> MSQIMYNYPAMLAHAAEMNTYSGALHAVGADIAAEQHALASAWQGDTGMTYQA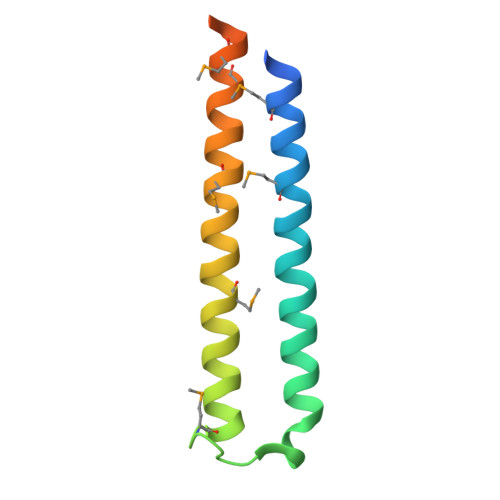WQAQWNQAMEELVRAYRAMATTHEQNTMAMSARDQAEGAKWGTHHHHHH>MTDTHTGPTPADAVPAYPFSLPHALDLDPHYAELRRDEPVSRVRLPYGEGTAWLVTRMSDARIVLGDSRFSTAAATDPATPRMFPTPPEPDGVLAQDPPDHTRLRRLVGKAFTARRVEEMRPRVRSLVDSLLDDMVAHGSPADLVEFLAVPFPVAVICELLGVPLEDRDLFRTFSDAMLSSTRLTAAEIQRVQQDFMVYMDGLVAQRRDAPTEDLLGALALATDNDDHLTKGEIVNMGVSLLIAGHETSVNQITNLVHLLLTERKRYESLVADPALVPAAVEEMLRYTPLVSAGSFVRVATEDVELSTVTVRAGEPCVVHFASANRDEEVFDHADELDFHRERNPHIAFGHGAHHCIGAQLGRLELQEALSALVRRFPTLDLAEPVAGLKWKQGMLIRGLERQIVSW[9x]

The bacterial P450 OleP, from Streptomyces antibioticus, is an epoxidase involved in the tailoring steps of the biosynthetic pathway of the antibiotic oleandomycin. More specifically, OleP catalyzes a regio- and stereospecific reaction of epoxidation at the C8-C8a of the macrolactone ring. Among the known macrolide epoxygenases from actinomycetes, OleP presents a unique epoxidation chemistry since it targets a non-activated C-C bond, which is a reaction not easily achievable through conventional chemical synthesis protocols. In addition, discordant findings have been reported concerning the timing of OleP activity during the tailoring phase of oleandomycin biosynthesis, showing that OleP is either active on the aglycone intermediate, 8.8a-deoxyoleandolide (DEO), or on the monoglycosylated one, L-olivosyl-8.8a-deoxyoleandolide (L-O-DEO).

As for OleP-6DEBLS, the crystal of OleP–DEOLS (ionic strength, I = 0.2 M) contains nine monomers in the asymmetric unit arranged in six open conformers and three closed ones. Therefore, in the presence of the physiological aglycone intermediate DEO, OleP can assume two conformational states, an open one (unproductive binding) and a closed one (productive binding). In the open active site, DEO assumes different orientations and conformations, but none of the six molecules of DEO expose the C8-C8a bond, which is the target of the OleP epoxidation, to the heme iron. The residues of the open OleP interacting with DEO are located on the BC loop (M83, F84, L94), on the N-terminus of the I helix (I243, A244, G245, E247, T248), on β-hairpin β3 (V291, G294, S295, F296) and on β-hairpin β4 (L396, I397). The functional groups that decorate the DEO macrolactone ring alternatively contact residues of the abovementioned set, depending on the position, the orientation, and the conformation adopted by DEO in the active site of each open monomer. Electron density accounting for the sixth coordinate water ligand, typical of a low spin enzyme, was observed in four out of six total open monomers. It is placed at about 2–2.5 Å distance from the heme iron and the substrate ligand, forming hydrogen bonds with the backbone carbonyl of A244 on helix I and with the aglycon substrate, involving the C1-carbonyl or the C3-OH or the C5-OH groups, depending on the monomer. A further interesting aspect that emerges from the structural analysis of OleP–DEO is that even the physiological aglycone substrate does not induce the closure of the OleP active site in the full population of the enzyme, at least in the OleP–DEOLS crystal form. As a consequence, efficient binding of DEO that induces the structural changes required to close OleP and to shift the iron-spin equilibrium to the high state, preparing it for catalysis, occurs on a small fraction of enzyme molecules as supported by having only one-third of the protein copies in the asymmetric unit of the OleP–DEOLS crystal form in the closed conformation.>MLRLKTQDSRLKTQDSRLKTQDSRLKTQDSFSVDDNGSGNVFVCGDLVNSKENKVQFNGNNNKLIIEDDVECRWLTVIFRGDNNYVRIHKNSKIKGDIVATKGSKVIIGRRTTIGAGFEVVTDKCNVTIGHDCMIARDVILRASDGHPIFDIHSKKRINWAKDIIISSYVWVGRNVSIMKGVSVGSGSVIGYGSIVTKDVPSMCAAAGNPAKIIKRNIIWARTDKAELISDDKRCSSYHAKLTQLEHHHHHH[3x]

O-acetylation of the E. coli K1 capsule is catalyzed by the acetyl-CoA dependent sialate O-acetyltransferase NeuO, an enzyme that is highly specific for α2,8-linked polySia with a minimum chain length of 14 residues. Beyond the variable poly-ψ-domain, NeuO is characterized by the presence of imperfect tandem repeats of the hexapeptide motif [LIV]-[GAED]-X2-[STAV]-X, a hallmark of the hexapeptide repeat family of acyltransferases. The crystal structures of several members of this family reveal that three hexapeptides fold into one coil of a left-handed parallel β-helix (LβH), which resembles a triangular prism. In this study, we have solved the structure of the prophage-encoded O-acetyltransferase NeuO responsible for phase-variable capsule modification of the neuroinvasive pathogen E. coli K1.

In the present study, we crystallized NeuO using a protein variant with four N-terminal RLKTQDS heptads. Protein expressed from the engineered sequence yielded crystals that belong to space group P21. The homotrimeric enzyme shares typical features of the LβH-family of acyltransferases combined with an unusual funnel-shaped outline. The predominant part of the NeuO monomer folds into an LβH-domain. However, in contrast to the canonical LβH fold, which resembles an equilateral triangular prism, the LβH domain of NeuO displays a more extended outline. Moreover, the parallel arrangement of the individual monomers is lost and the monomers are arranged with a notable inclination of 45° and 34° between each chain in NeuO and OatWY, respectively. Despite close intersubunit interactions at the bottom of the trimer, a tunnel can be observed between each subunit. However, since the poly-ψ-domain is not visible in the electron density of the crystal structure it can be concluded that it is disordered in the apo-enzyme. Albeit the structure of the first 18 residues could not be solved for the apo-enzyme, the overall outline of NeuO with the N-termini of the three subunits pointing almost 65 Å away from each other, exclude the formation of a triple coiled-coil. The structural data show that both residues are located in the proposed active site in positions highly conserved among acetyltransferases of the LβH family (MAT, GAT, VatD, PaXAT, and OatWY).MOENOMYCIN | C69 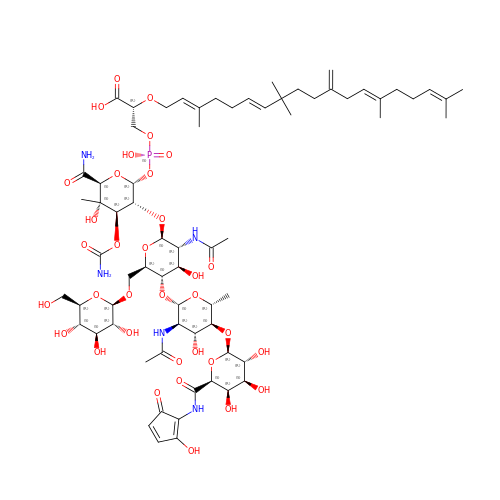H106 N5 O34 P | NXPRJQIAIORCGO-ZLPAOQQDSA-N> MGSTEQSIQLTLGPWYSNDGKYSNPTIPVYTIQKTRSDTENMVVVVCGEGYTKSQQGKFINDVKRLWQDAMKYEPYRSYADRFNVYALCTASESTFDNGGSTFFDVIVDKYNSPVISNNLHGSQWKNHIFERCIGPEFIEKIHDAHIKKKCDPNTIPSGSEYEPYYYVHDYIAQFAMVVNTKSDFGGAYNNREYGFHYFISPSDSYRASKTFAHAFGHGLLGLGDEYSNGYLLDDKELKSLNLSSVEDPEKIKWRQLLGFRNTYTCRNAYGSKMLVSSYECIMRDTNYQFCEVCRLQGFKRMSQLVKDVDLYVATPEVKEYTGAYSKPSDFTDLETSSYYNYTYNRNDRLLSGNSKSRFNTNMNGKKIELRTVIQNISDKNARQLKFKMWIKHSDGSVATDSSGNPLQTVQTFDIPVWNDKANFWPLGALDHIKSDFNSGLKSCSLIYQIPSDAQLKSGDTVAFQVLDENGNVLADDNTETQRYTTVSIQYKFEDGSEIPNTAGGTFTVPYGTKLDLTPAKTLYDYEFIKVDGLNKPIVSDGTVVTYYYKNLEHHHHHH

The sole known peptidase capable of cleaving both IgA1 and IgA2 is IgAse, a unique enzyme encoded by Thomasclavelia ramosa (formerly Clostridium ramosum). IgAse is a ~ 140-kDa, seven-domain, membrane-bound metallopeptidase (MP). Differential scanning fluorimetry, small-angle X-ray scattering, AI-based structural predictions, mass spectrometry, and high-resolution crystallography and cryo-electron microscopy of multidomain fragments of IgAse revealed a novel 313-residue catalytic domain (CD) from the igalysin family within the metzincin MP clan. The CD is flanked by an N-terminal globular C-type lectin-like domain and a wrapping domain (WD), followed by four all-β domains.

Recombinant production and biophysical assessment of IgA1, IgA2 and IgAse — To investigate the interplay between IgAse and IgA, we cloned a panel of seven peptidase constructs, which included the wild-type CD and the inactive E540A-variant, in which the glutamate acting as general base/acid for catalysis in most MPs (hereafter “catalytic glutamate”) was replaced with alanine. The crystals were densely packed, containing 42% solvent compared to the average 51% for protein crystals, which accounts for the high resolution of the diffraction data and the resulting Fourier maps (1.75 Å). Two search models derived from the prediction in Section 3.1 were used, corresponding to domains CD + WD (N331–N807) and Oβ (R808–N876), respectively. These calculations, which identified P21 as the correct space group, yielded a unique solution for either moiety, corresponding to a single IgAse protomer in the asymmetric unit (a.u.). The final structure encompasses IgAse residues E330–N876, plus a leucine from the C-terminal purification tag, two zinc cations, a tetraethylene glycol molecule, eight ethylene glycol molecules, and 430 solvent molecules. In addition, a formate anion, which is a metabolite of the E. coli expression host potentially taken up by IgAse during heterologous overexpression, was tentatively assigned attached to the catalytic zinc. The CD is asymmetrically divided into a larger upper subdomain (USD; E330–L546) and a smaller lower subdomain (LSD; G547–V634) by a horizontal, deep active-site cleft that traverses the entire domain and extends from the non-primed to the primed side in the standard orientation of MPs. Moreover, the third ligand in IgAse is also an aspartate (D550), resulting in a unique zinc motif (H539E540xxH543xxxG547xxD550). Consequently, the WD sandwich functions as a scaffold, positioning the two flaps as clamps that reach around and thus stabilize the CD.> SDTAPAGFQLEKVVILSRHGVRAPTKMTQTMRDVTPHQWPEWPVKLGYITPRGEHLISLMGGFYRERFQQQGLLPKDNCPTPDAVYVWADVDQRTRKTGEAFLAGLAPQCDLAIHHQQNTQQADPLFHPVKAGICSMDKSQVHAAVEKQAGTPIETLNQRYQASLALMSSVLDFPKSPYCQQHNIGKLCDFSQAMPSRLAINDDGNKVALEGAVGLASTLAEIFLLEHAQGMPKVAWGNIHTEQQWNSLLKLHNAQFDLMSRTPYIAKHNGTPLLQTIAHALGSNITSRPLPDISPDNKILFIAGHDANIANISGMLGMTWTLPGQPDNTPPGGALVFERWVDNAGKPYVSVNMVYQTLAQLHDQAPLTLQHPAGSVRLNIPGCSDQTPDGYCPLSTFSRLVSHSVEPACQLP

Phytases (myo-inositol hexakisphosphate phosphohydrolases) catalyse the hydrolysis of phytate into inorganic phosphate (Pi) and lower phosphorylated myo-inositols. Here we report the identification of two HAPPs from the enterobacteria Hafnia alvei (HaPhy) and Yersinia kristensenii (YkPhy), together with biochemical studies of their pH and temperature optima, as well as their phytate degradation pattern, which show that they are 6-phytases. The enzymes share a common catalytic site architecture located at the interface of the two domains involving the conserved N-terminal active site motif RHGXRXP and the C-terminal HD. The two-step reaction involves a nucleophilic attack on the phosphorous by the histidine from the RHGXRXP motif to form a covalent phosphohistidine intermediate while the aspartic acid of the HD motif serves as a proton donor to the oxygen atom of the scissile phosphomonoester bond.

The MIHS-HaPhy complex is the first structure of a 6-phytase showing a phytate analogue with the 6-position in the catalytic site. Co-crystals with the wild-type HaPhy grew in clusters of insufficient quality for data collection, but a successful hit was obtained for the 5% active T308A mutant of the enzyme. While the mutant MIHS-HaPhy complex crystallised in a different space group to the apo-enzyme and tar-HaPhy complex, the overall fold is essentially unchanged, with one molecule in the asymmetric unit and residues 184–189 disordered. MIHS is coordinated by Arg18, His19, Arg22, Thr25, Lys26, His128, Thr219, His306, Asp307 and a number of water molecules. The Nε2 atom of the catalytic nucleophile, His19, lies 3.2 Å from S6 of the MIHS and is in-line with the S-O bond from the inositol ring. The OD1 atom of Asp307, the proton donor, forms an H-bond with the oxygen at position 6 of the inositol ring, Fig. 5b,c,d. Thr308 has been mutated to alanine in the MIHS-HaPhy complex, so a potential H-bond to the 1-sulphate is missing: Thr305, the equivalent residue in EcPhy, coordinates the axial 2-phosphate. There is a second MIHS bound between three symmetry-related phytase molecules in the crystal, in a completely different conformation, with the 2-sulphate in the equatorial orientation and all five others axial. A key feature is the presence of a potassium ion, coordinated by four oxygens from three sulphates of the MIHS (1, 3 and 5) with its ligand shell completed by the main chain oxygens of Gly230 and Gly231.> KDTIALVVSTLNNPFFVSLKDGAQKEADKLGYNLVVLDSQNNPAKELANVQDLTVRGTKILLINP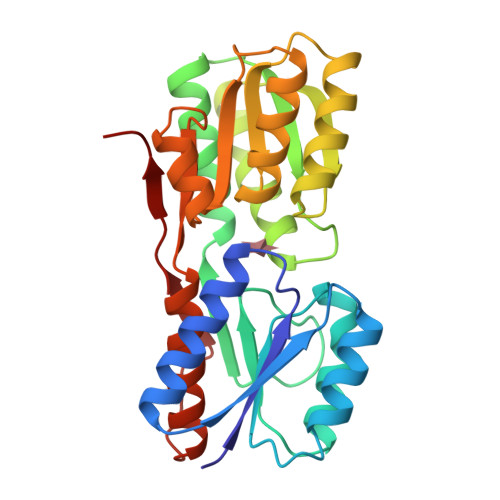TDSDAVGNAVKMANQANIPVITLDRQATKGEVVSHIASDNVLGGKIAGDYIAKKAGEGAKVIELQGTAATSAARERGEGFQQAVAAHKFNVLASQPADFDRIKGLNVMQNLLTAHPDVQAVFAQNDEMALGALRALQTAGKSDVMVVGFDGTPDGEKAVNDGKLAATIAQLPDQIGAKGVETADKVLKGEKVQAKYPVDLKLVVKQ> GSMDALEGESFALSFSSASDAEFDAVVGYLEDIIMDDEFQLLQRNFMDKYYLEFEDTEENKLIYTPIFNEYISLVEKYIEEQLLQRIPEFNMAAFTTTLQHHKDEVAGDIFDMLLTFTDFLA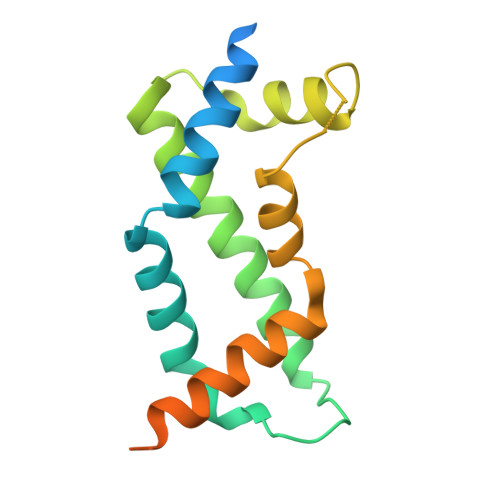FKEMFLDYRAEKEGRGLDLSSGLVVTSLCKSSSLPASQNNLRH> MASSLAQQLAQIAANSRSSFNVKALKASHSKSLIWEPRVAVSQTFAEIYSQCYEGFKELCHLDSRFVPFDATLFSAQSQEVDRTQMTAEENAALDKRVDSFLHLVGSRLRLMPAIKAVEWLIRRFRIHEFNTGTLLATFLPYHTIPAFVTLLSILPVQRIPIEYRFLDPYIKSLTPPPRAAIVQQATNRPDLLSAISRYTLDSCRAKQEYPGLISFWGGIMAEAVNGMIDKMRSGRRAIQLENDHL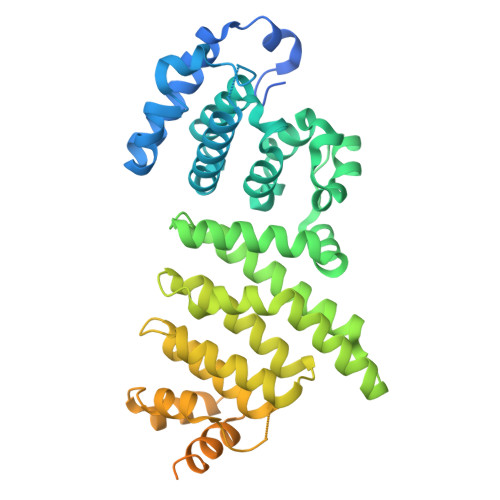LLQQIGPVLSEAMVMKDVPGIQIASYMVVAILAAKGSLNDNILTAFMEQLVHGWTVDTLRPGLVCLTMLAQHRSAKQLSGRVAKAVIKVPDLVSSLRDISKEHQVDKLANGLVLAFVDRLAKKGDIRTLPVINSLLLSELLQEKQAKVAYKALLLAAHKIDDNVDADGNIRKQVGSALVRLSQAEGDVGDAIRTAIQEVDFNIEELELKLGAAIRPKLAIEEAPE>[2x]MVLYFIGLGLYDERDITVKGLEIAKKCDYVFAEFYTSLMAGTTLGRIQKLIGKEIRVLSREDVELNFENIVLPLAKENDVAFLTPGDPLVATTHAELRIRAKRAGVESYVIHAPSIYSAVGITGL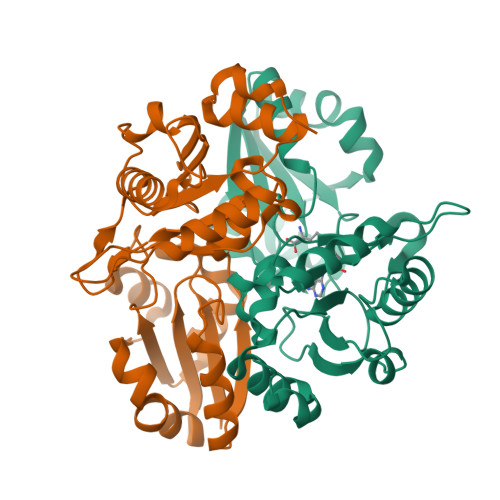HIYKFGKSATVAYPEGNWFPTSYYDVIKENAERGLHTLLFLDIKAEKRMYMTANEAMELLLKVEDMKKGGVFTDDTLVVVLARAGSLNPTIRAGYVKDLIREDFGDPPHILIVPGKLMIVEAEYLVEIAGAPREILRVNV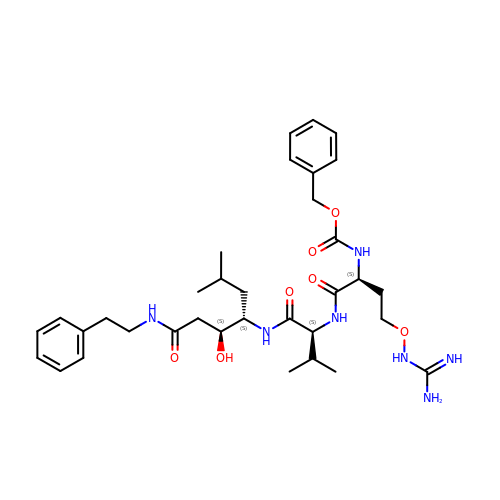N-[(benzyloxy)carbonyl]-O-carbamimidamido-L-homoseryl-N-{(3S,4S)-3-hydroxy-6-methyl-1-oxo-1-[(2-phenylethyl)amino]heptan-4-yl}-L-valinamide | C34 H51 N7 O7 | VAHRPHLZONNTFF-NUISNXNRSA-N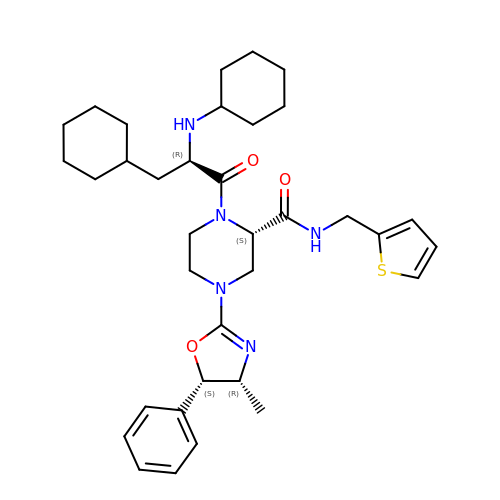(2S)-1-(N,3-dicyclohexyl-D-alanyl)-4-[(4R,5S)-4-methyl-5-phenyl-4,5-dihydro-1,3-oxazol-2-yl]-N-[(thiophen-2-yl)methyl]piperazine-2-carboxamide | C35 H49 N5 O3 S | CTYNKFLWABFRHE-BESSAKRQSA-N>GVSLRKAERLRAELLDLKAGGFSIRNQ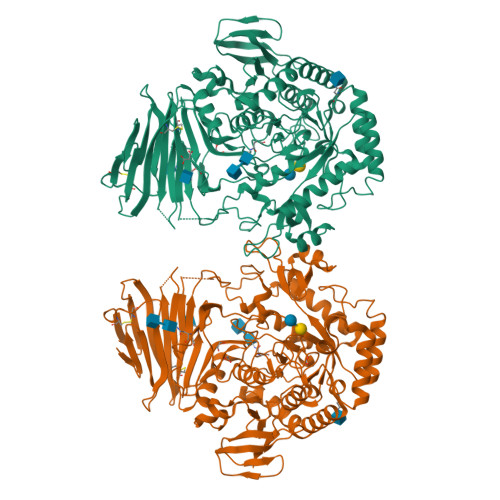KGEQVFRLAFRSGALDLDSCSRDGALLGCSLTADGLPLHFFIQTVRPKDTVMCYRVRWEEAAPGRAVEHAMFLGDAAAHWYGGAEMRTQHWPIRLDGQQEPQPFVTSDVYSSDAAFGGILERYWLSSRAAAIKVNDSVPFHLGWNSTERSLRLQARYHDTPYKPPAGRAAAPELSYRVCVGSDVTSIHKYMVRRYFNKPSRVPAPEAFRDPIWSTWALYGRAVDQDKVLRFAQQIRLHHFNSSHLEIDDMYTPAYGDFDFDEVKFPNASDMFRRLRDAGFRVTLWVHPFVNYNSSRFGEGVERELFVREPTGRLPALVRWWNGIGAVLDFTHPKARDWFQGHLRRLRSRYSVASFKFDAGEVSYLPRDFSTYRPLPDPSVWSRRYTEMALPFFSLAEVRVGYQSQNISCFFRLVNRDSVWGYDLGLRSLIPAVLTVSMLGYPFILPDMVGGNAVPQRTAGGDVPERELYIRWLEVAAFMPAMQFSIPPWRYDAEVVAIAQKFAALRASLVAPLLLELAGEVTDTGDPIVRPLWWIAPGDETAHRIDSQFLIGDTLLVAPVLEPGKQERDVYLPAGKWRSYKGELFDKTPVLLTDYPVDLDEIAYFTWAS[4x]> VASTMTDG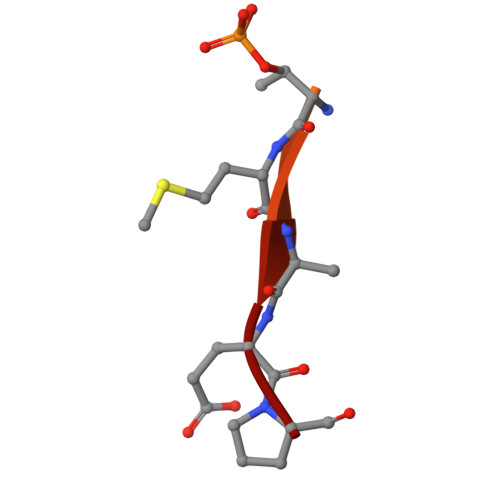ANTMIEP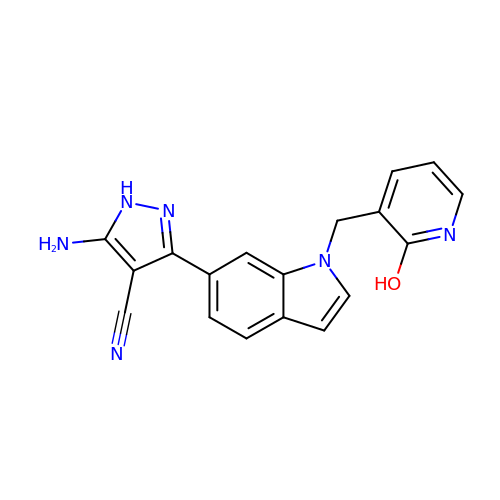5-azanyl-3-[1-[(2-oxidanylpyridin-3-yl)methyl]indol-6-yl]-1~{H}-pyrazole-4-carbonitrile | C18 H14 N6 O | RTLAMMYDMUSFRK-UHFFFAOYSA-N> HHHHHHMPVFHTRTIESILEPVAQQISHLVIMHEEGEVDGKAIPDLTAPVAAVQAAVSNLVRVGKETVQTTEDQILKRDMPPAFIKVENACTKLVQAAQMLQSDPYSVPARDYLIDGSRGILSGTSDLLLTFDEAEVRKIIRVCKGILEYLTVAEVVETMEDLVTYTKNLGPGMTKMAKMIDERQQELTHQEHRVM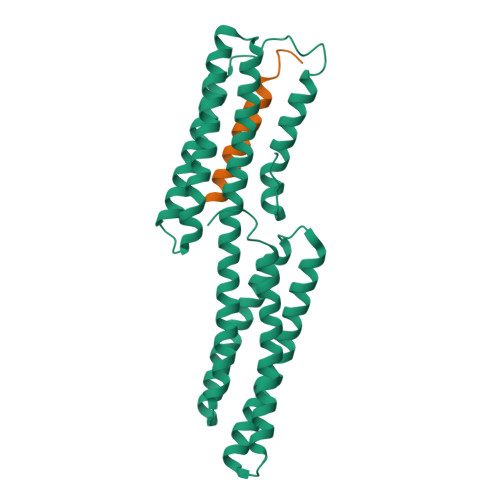LVNSMNTVKELLPVLISAMKIFVTTKNSKNQGIEEALKNRNFTVEKMSAEINEIIRVLQLTSWDEDAW;> PLLQAAKGLAGAVSELLRSAQPASA In mammals, the canonical Hippo pathway contains a core kinase cascade, formed by STE20-like MST1/2 kinases, Large Tumor Suppressor LATS1/2 kinases, the WW-domain containing scaffold protein Salvador (SAV1) and the adaptor protein MOB1. MST1/2 contain an N-terminal kinase domain and a C-terminal coiled-coil SARAH domain, which are separated by a flexible linker. MST1 and MST2 can each form a constitutive homodimer through the SARAH domain, and kinase activation is achieved by trans-autophosphorylation of the activation loop (T183 for MST1 and T180 for MST2). In this study, using a combination of biochemical, structural, and cell biological experiments, we establish the PP2A complex, STRIPAKSLMAP, as a key negative regulator of Hippo signaling in human cells, and show that SAV1 promotes MST1/2 activation through antagonizing the STRIPAKSLMAP PP2A phosphatase activity.

To understand how SAV1 activates MST2, we determined the crystal structure of MST2 ∆L/D146N bound to the SARAH domain of SAV1 (residues 291–383). Surprisingly, MST2–SAV1 does not form an expected heterotetramer through a four-helix bundle formed by their SARAH domains. Instead, SAV1 SARAH and MST2 SARAH form a heterodimer, similar to that formed by the SARAH domains of MST2 and one of the RASSF family of tumor suppressors, RASSF5. The active site of MST2 in MST2–SAV1 is well-defined. The Mg2+ ion and AMP-PNP are clearly visible in the electron-density map. The MST2 kinase domain in MST2–SAV1 is structurally very similar to the MST2 kinase alone, except that the T-loop helix observed in the MST2 kinase structure is not visible in the MST2–SAV1 structure. The K56-E70 salt bridge between strand β3 and helix αC is not formed in MST2–SAV1, consistent with MST2 adopting the inactive conformation. The SARAH domains of MST2 and SAV1 form a long antiparallel coiled coil and do not directly contact the kinase domain. The N-terminal extension of SAV1 SARAH forms two short helices, H0 and H1, which interact with the main coiled coil through several hydrophobic interactions. Furthermore, the SAV1- and RASSF5-binding surfaces of MST2 SARAH are virtually identical, readily explaining mutually exclusive binding of SAV1 and RASSF5 to MST2.

> EDSLTKQPEEVFDVLEKLGEGSYGSVFKAIHKESGQVVAIKQVPVESDLQEIIKEISIMQQCDSPYVVKYYGSYFKNTDLWIVMEYCGAGSVSDIIRLRNKTLIEDEIATILKSTLKGLEYLHFMRKIHRNIKAGNILLNTEGHAKLADFGVAGQLTDTMAKRNTVIGTPFWMAPEVIQEIGYNCVADIWSLGITSIEMAEGKPPYADIHPMRAIFMIPTNPPPTFRKPELWSDDFTDFVKKCLVKNPEQRATATQLLQHPFIKNAKPVSILRDLITEAMEIKAKRHEEQQRELEEEENWKVPQDGDFDFLKNLSLEELQMRLKALDPMMEREIEELRQRYTAKRQPILDAMDAKKRRQQNF;> SLLVPANPYHTAEIPDWLQVYARAPVKYDHILKWELFQLADLDTYQGMLKLLFMKELEQIVKMYEAYRQALLTELENRKQRQQWYAQQHGKNF>MGSITENTSWNKEFSAEAVNGVFVLCKSSSKSCATNDLARASKEYLPASTFCIPNAIIGLETGVIKNEHQVFKWDGKPRAMKQWERDLTLRGAIQVSAVPVFQQIAREVGEVRMQKYLKKFSYGNQNISGGIDKFWLEGQLRISAVNQVEFLESLYLNKLSASKENQLIV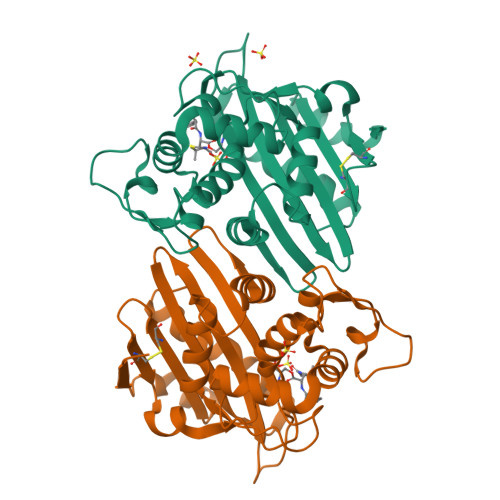KEALVTEAAPEYLVHSKTGFSGVGTESNPGVAWWVGWVEKETEVYFFAFNMDIDNESKLPLRKSIPTKIMESEGIIGG[2x]L-PROLINE, 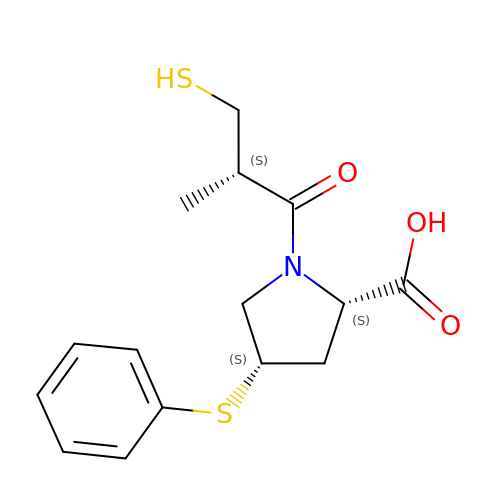1-[(2S)-3-MERCAPTO-2-METHYL-1-OXOPROPYL]-4-(PHENYLTHIO)-, 4S | C15 H19 N O3 S2 | UQWLOWFDKAFKAP-WXHSDQCUSA-N>MASDESMVP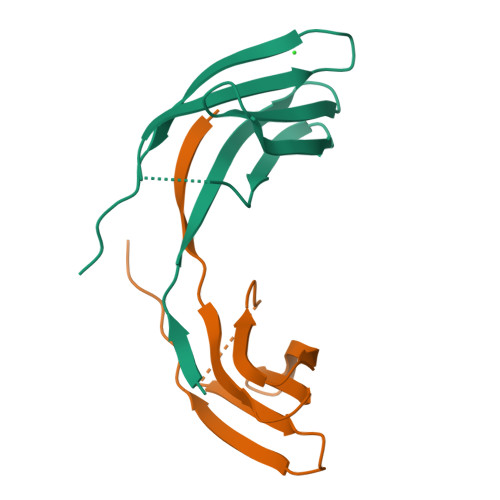YYQWNFAPVVRGIARTQARVEVLRDGYTVSNELVPSGPFELANLPLGGGSGELKVIIHESDGTKQVFTVPYDTPAVALRKG[2x]> PVMHPHGVPPSHRPWQMKDLQAIKQEVSQAAPGSPQFMQTIRLAVQQFDPTAKDLQDLLQYLCSSLVASLHHQQLDSLISEAETRGITGYNPLAGPLRVQANNPQQQGLRREYQQLWLTAFAALPGS

Human T-cell Leukaemia Virus type 1 (HTLV-1) is an untreatable retrovirus that causes lethal malignancies and degenerative inflammatory conditions. Here, we show that high-resolution crystal structures of the mature-length HTLV-1c CA protein define essential lattice interfaces and identify a distinct ligand-binding pocket. Across the known Orthoretrovirinae, CA is a two-domain protein with HIV being the best characterised. However, our structures reveal that HTLV-1 does still have a pocket formed between helices 3, 4, and 5, albeit an electropositive one capable of binding to either phosphate or sulfate in vitro.

As sulfate is unlikely to be relevant to the HTLV infectious process, we performed a similar soak with sodium/potassium phosphate, obtaining a phosphate-bound structure to an almost identical resolution (1.73 Å). Interestingly, in crystallants at physiological pH, we observed partial occupancy of both sulfate and phosphate, while full occupancy was achieved under acidic conditions (pH 6 and below). This phenomenon likely reflects the protonation state of the binding pocket, which includes two histidine sidechains (H71 and H72) that typically gain positive charge under acidic conditions. Unlike FG-cofactor or drug binding in HIV, phosphate/sulfate binding in HTLV-1c results in significant structural changes, especially at residues H72 and R98. One possible explanation would be that a bound cofactor is required for appropriate immature lattice formation prior to budding. It is particularly striking that H72 is so conformationally responsive to sulfate/phosphate binding, while also participating in the trimer interface, and also being essential for infectivity and particle production. Mutants that would remove a direct interaction with the sulfate or phosphate groups (H71A, H72A, R98A and W117A) all effectively abolished infectivity with a concomitant loss of particle production. In the HTLV-1 case, sulfate is unlikely to be the endogenous cofactor, and inorganic phosphate is too ubiquitous to provide any spatiotemporal regulation to the capsid but could potentially function as a ‘pocket factor’. A cryptic phosphopeptide, on the other hand, could conceivably function as a capsid-binding cofactor at this site.>[2x]MEITPSDVIKTLPRQEFSLVFQKVKEMEKTGAHIINLGQGN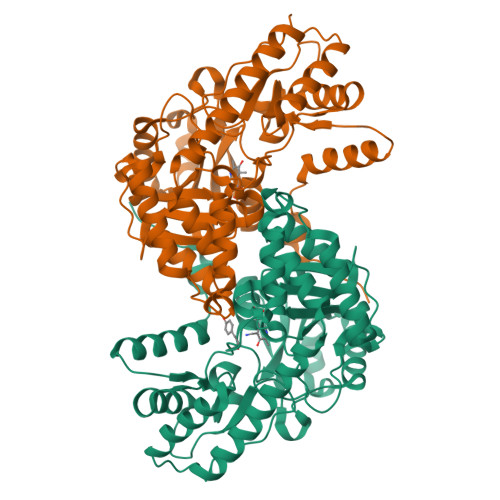PDLPTPPHIVEALREASLNPSFHGYGPFRGYPFLKEAIAAFYKREYGVTINPETEVALFGGGKAGLYVLTQCLLNPGDIALVPNPGYPEYLSGITMARAELYEMPLYEENGYLPDFEKIDPAVLEKAKLMFLNYPNNPTGAVADAAFYAKAAAFAKEHNIHLIHDFAYGAFEFDQKPASFLEAEDAKTVGAELYSFSKTFNMAGWRMAFAVGNEKIIQAVNEFQDHVFVGMFGGLQQAASAALSGDPEHTESLKRIYKERIDFFTALCEKELGWKMEKPKGTFYVWAEIPNTFETSHQFSDYLLEHAHVVVTPGEIFGSNGKRHVRISMVSKQEDLREFVTRIQKLNLPFGSLQETSR> MPQDPSTRSSPARLLIPEPRAGRARHAACVLLAVCFVVLFLSGEPLAPIIRSVCTQLAALQLGVLLKGCCCLAEEIFHLHSRHHGSLWQVLCSCFPPRWYLALLLVGGSAYLDPPEDNGHSPRLALTLSCLCQLLVLALGLQKLSAVEVSELTESSKKNVAHGLAWSYYIGYLKVVLPRLKECMEELSRTNPMLRAHRDTWKLHILVPLGCDIWDDLEKADSNIQYLADLPETILTRAGIKRRVYKHSLYVIRDKDNKLRPCVLEFASPLQTLCAMSQDDCAAFSREQRLEQARLFYRSLRDILGSSKECAGLYRLIAYEEPAEPESHFLSGLILWHLQQQQREEYMVQEELPLGTSSVELSLQV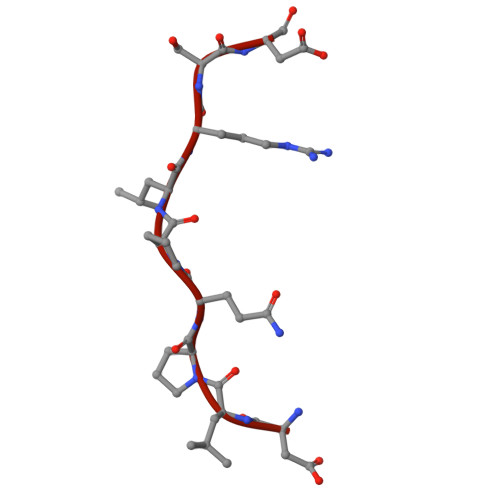SSSDLPQPLRSDCPGIHRPDYKDDDDK> MSGYSNPLNDPIMIRTMIVYGNLSATYFTGNGAALTQQPIASNVPPTLRADAFGNVTSPANVISGNITTIDVISAGNINTRYVFGDGSTLSGISTGNSVVGVQKIDIIGNAVSSTISTGSLRTNVAFTNITANISNISYLSGNTVSNIINASNLIANIVNANVMSGDITLNRIVATDTRTINLFGNVSTNSFTAYGNVTANILTATTLTANSLQIESVSGNSVQKMIVGNLIGNVLTARTATFDTANIPTITSNVGIFTVANIRTITGDVRANVLNVSNIVTRSIGTDVVSNNIIATIGNVQSMIIGNLSANTLSVSNGTFQNFTTTVGLNVTTLSASVSNALVLSFTTGNSSSTTTTNLDAYGNTQFLRISTETSGINILNANSVSVGNLTIVGNVTSTSNNISGQVTSNSSQVQNINTNVIYSGNVFTSRFIAANANIRSLTASIGQVNSLTITSGNLTSLSFVNGNGNGVIATNANISNLNAVSMSGFAFDA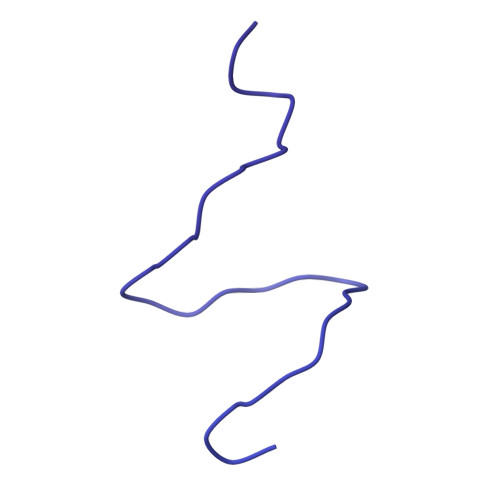NVIIGDITANILSSGNLNANVFEANMLTSGNVVSTNGDTGTINANSIVLNVISGGDTRIDRLIANSVTTGDFYTTSTITAGVIDCAQGKISGNSSSNASLISNVISANTASFVNTSVGYGNLVNAVVIGNIIANVVTSGDANAVFLNSNLTTSGSIFGNISNSASIVAEYSNIRTMNVGNINSTTFNAEYLYVGNITVTGVSNTGYLICRNATFSLNSNIQTLITENVTTSNAGSNIFTNVITTGNAFSQNINTINANVLGITSVFSNVITNISNIRTLILLSNVSLGNLTATSANVTSNVSVGNLIGNIVASNAFFNTATIRNLAIFDVTGNILVAQSNASISNLTTERILLSDANIANLSTSNVSSNIAVVTGTCRIDAINSSNITFTNTATVSAAVVNVLGNLTVSNVINVQNLTANVGNIWQAVSNIQSMTTANIFTNTMTIINSFTYSNISSQRLIATNTLTANGVNLFSNIANLTVSGNANVGRWIAASAPATGALCFSSTESANLTTANLFAGNLNTWRAFVGNVIGNVMTTVAGDFGGIRVSVANIDVSGVANVENFTVNGNLFATNVITRDLSANLINFSGSLSNTSSISISGNSLFTSSANAANVGVSINMITQNLFGNRLSSENIQGNVLQASNIAVSQTVNVVGNISIGNLSVSRELFANSITISSGGTIVGNNTTRMITTPTSNSWSVGSLVGNANVSVQFTANTMVVQNIQPNTLVVNINQSTPTSNSGVRAIYIGYIVPVNFNATSSTTVSFSPALPTNCIYMPQLQYYSGGTVLQNNASFSTQIGLGVETITNTSCTIRMSTLDTLPIPSTSFFGLMVTAVQTV>[2x]GMSGSRPTQSSEGSRRSRHSARIIAQTTVDAKLHADFEESGSSFDYSTSVRVTGPVVENQPPRSDKVTTTYLHHIQKGKLIQPFGCLLALDEKTFKVIAYSENASELLTMASHAVPSVGEHPVLGIGTDIRSLFTAPSASALQKALGFGDVSLLNPILVHCRTSAKPFYAIIHRVTGSIIIDFEPVKPYEVPMTAAGALQSYKLAAKAITRLQSLPSGSMERLCDTMVQEVFELTGYDRVMAYKFHEDDHGEVVSEVTKPGLEPYLGLHYPATDIPQAARFLFMKNKVRMIVDCNAKHARVLQDEKLSFDLTLCGSTLRAPHSCHLQYMANMDSIASLVMAVVVNEEDGEGDAPDATTQPQKRKRLWGLVVCHNTTPRFVPFPLRYACEFLAQVFAIHVNKEVELDNQMVEKNILRTQTLLCDMLMRDAPLGIVSQSPNIMDLVKCDGAALLYKDKIWKLGTTPSEFHLQEIASWLCEYHMDSTGLSTDSLHDAGFPRALSLGDSVCGMAAVRISSKDMIFWFRSHTAGEVRWGGAKHDPDDRDDARRMHPRSSFKAFLEVVKTRSLPWKDYEMDAIHSLQLILRNAFKDSETTDVNTKVIYSKLNDLKIDGIQELEAVTSEMVRLIETATVPILAVDSDGLVNGWNTKIAELTGLSVDEAIGKHFLTLVEDSSVEIVKRMLENALEGTEEQNVQFEIKTHLSRADAGPISLVVNACASRDLHENVVGVCFVAHDLTGQKTVMDKFTRIEGDYKAIIQNPNPLIPPIFGTDEFGWCTEWNPAMSKLTGLKREEVIDKMLLGEVFGTQKSCCRLKNQEAFVNLGIVLNNAVTSQDPEKVSFAFF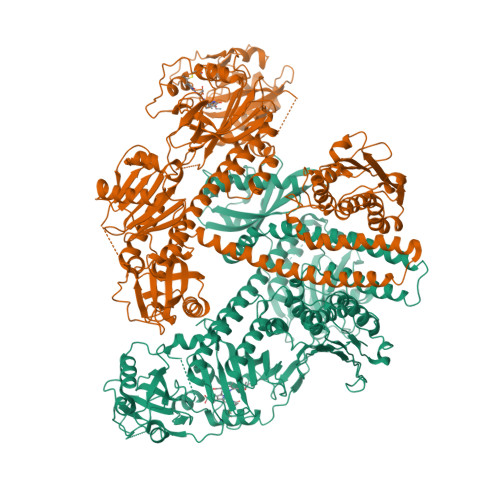TRGGKYVECLLCVSKKLDREGVVTGVFCFLQLASHELQQALHVQRLAERTAVKRLKALAYIKRQIRNPLSGIMFTRKMIEGTELGPEQRRILQTSALCQKQLSKILDDSDLESIIEGCLDLEMKEFTLNEVLTASTSQVMMKSNGKSVRITNETGEEVMSDTLYGDSIRLQQVLADFMLMAVNFTPSGGQLTVSASLRKDQLGRSVHLANLEIRLTHTGAGIPEFLLNQMFGTEEDVSEEGLSLMVSRKLVKLMNGDVQYLRQAGKSSFIITAELAAANK> MANENILKLKLYRSLGVILDLENDQVLINRKNDGNIDILPLDN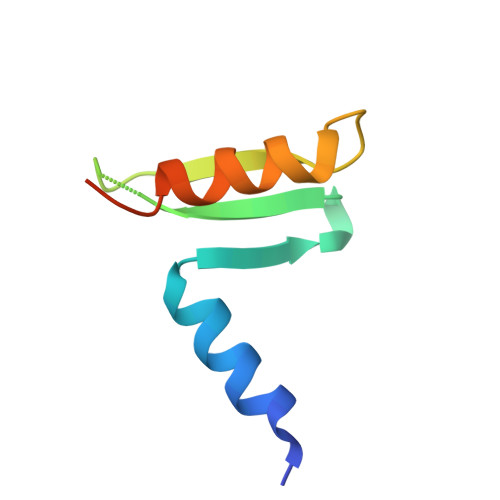NLSDFYKTKYIWERLGKHHHHHH> XKVKQLKAKVEELKSKLWHLKNKV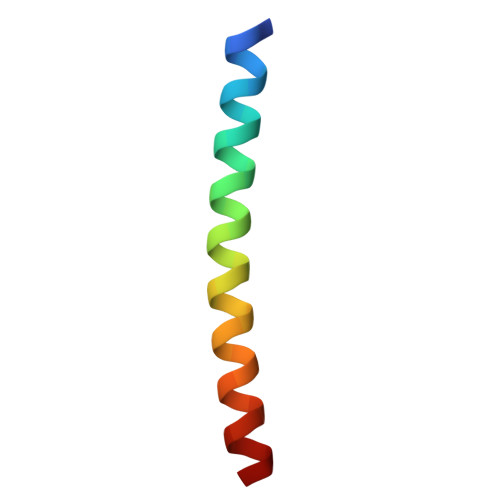ARLKKKNAECKA> ASVLWFQGGACSGNTMSFLNADEPNVVDLIVDFGLDLLWHPSLGLELGNNAQKVFWDCAKGERPLDIFVFEGTVIEAPNGTGQMDMFAGRPMKDWVTDLAGAAQIVVAIGDCACFGGIPAMEPNPSGSTGLQFHKREKGGFLGPDFRSKMGLPVINVPGCPAHPDWITQILVALATGRA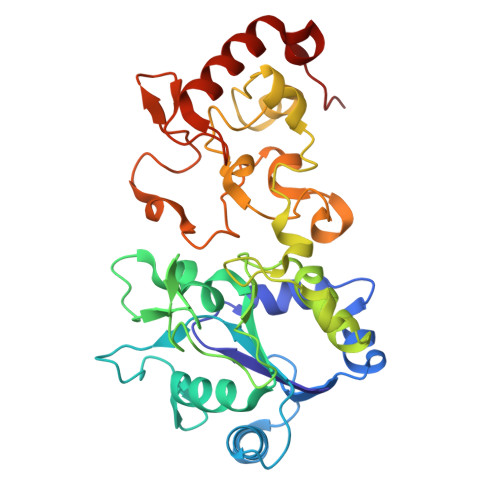GDITLDDLHRPETFFKTFTQTGCTRVQFFEYKQSTLSFGEGTRTGCLFYEFGCRGPMTHSPCNRILWNRQSSKTRAGMPCLGCTEPEFPHFDLAPGTVFKTQKVSGMIPKEVPEGTDHLTYMGLAAAARIAAPQWSKEDMFVV> X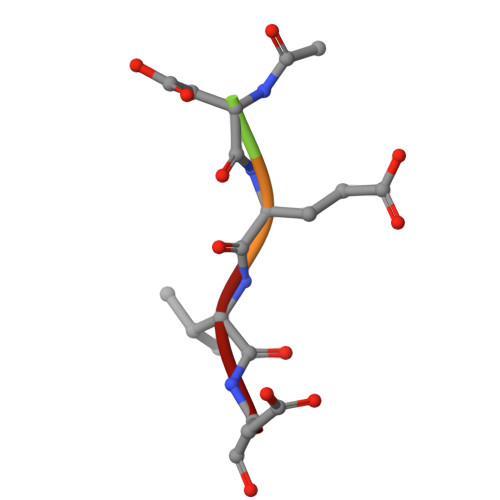DEVD> MASDYKDDDDKGALEVLFQGPSSPMAGNLVSWACKLCRSPEGFGPISFYGDFTQCFIDGVILNLSAIFMITFGIRDLVNLCKKKHSGIKYRRNWIIVSRMALVLLEIAFVSLASLNISKEEAENFTIVSQYASTMLSLFVALALHWIEYDRSVVANTVLLFYWLFETFGNFAKLINILIRHTYEGIWYSGQTGFILTLFQVITCASILLLEALPKKPLMPHQHIHQTLTRRKPNPYDSANIFSRITFSWMSGLMKTGYEKYLVEADLYKLPRNFSSEELSQKLEKNWENELKQKSNPSLSWAICRTFGSKMLLAAFFKAIHDVLAFTQPQLLRILIKFVTDYNSERQDDHSSLQGFENNHPQKLPIVRGFLIAFAMFLVGFTQTSVLHQYFLNVFNTGMYIKSALTALIYQKSLVLSNEASGLSSTGDIVNLMSVDVQKLQDLTQWLNLIWSGPFQIIICLYSLYKLLGNSMWVGVIILVIMMPLNSFLMRIQKKLQKSQMKYKDERTRVISEILNNIKSLKLYAWEKPYREKLEEVRNNKELKNLTKLGCYMAVTSFQFNIVPFLVSCCTFAVFVYTEDRALTTDLVFPALTLFNLLSFPLMIIPMVLNSFIEASVSIGRLFTFFTNEELQPDSVQRLPKVKNIGDVAINIGDDATFLWQRKPEYKVALKNINFQAKKGNLTCIVGKVGSGKTALLSCMLGDLFRVKGFATVHGSVAYVSQVPWIMNGTVKENILFGHRYDAEFYEKTIKACALTIDLAILMDGDKTLVGEKGISLSGGQKARLSLARAVYARADTYLLDDPLAAVDEHVARHLIEHVLGPNGLLHTKTKVLATNKVSALSIADSIALLDNGEITQQGTYDEITKDADSPLWKLLNNYGKKNNGKSNEFGDSSESSVRESSIPVEGELEQLQKLNDLDFGNSDAISLRRASDATLGSIDFGDDENIAKREHREQGKVKWNIYLEYAKACNPKSVCVFILFIVISMFLSVMGNVW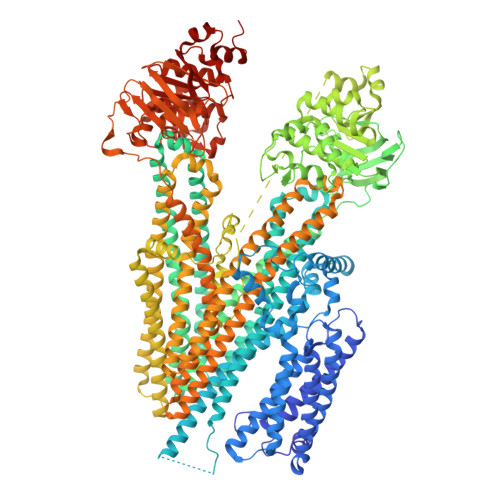LKHWSEVNSRYGSNPNAARYLAIYFALGIGSALATLIQTIVLWVFCTIHASKYLHNLMTNSVLRAPMTFFETTPIGRILNRFSNDIYKVDALLGRTFSQFFVNAVKVTFTITVICATTWQFIFIIIPLSVFYIYYQQYYLRTSRELRRLDSITRSPIYSHFQETLGGLATVRGYSQQKRFSHINQCRIDNNMSAFYPSINANRWLAYRLELIGSIIILGAATLSVFRLKQGTLTAGMVGLSLSYALQITQTLNWIVRMTVEVETNIVSVERIKEYADLKSEAPLIVEGHRPPKEWPSQGDIKFNNYSTRYRPELDLVLKHINIHIKPNEKVGIVGRTGAGKSSLTLALFRMIEASEGNIVIDNIAINEIGLYDLRHKLSIIPQDSQVFEGTVRENIDPINQYTDEAIWRALELSHLKEHVLSMSNDGLDAQLTEGGGNLSVGQRQLLCLARAMLVPSKILVLDQATAAVDVETDKVVQETIRTAFKDRTILTIAHRLNTIMDSDRIIVLDNGKVAEFDSPGQLLSDNKSLFYSLCMEAGLVNENGLVPRGSSAHHHHHHHHHHGA> MSLSEIKHWVFDMDGTLTIAVHDFAAIREALSIPAEDDILTHLAALPADESAAKHAWLLEHERDLAQGSRPAPGAVELVRELAGRGYRLGILTRNARELAHVTLEAIGLADCFAEADVLGRDEAPPKPHPGGLLKLAEAWDVSPSRMVMVGDYRFDLDCGRAAGTRTVLVNLPDNPWP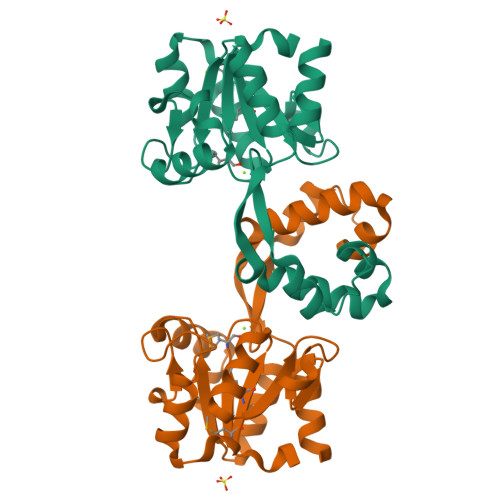ELTDWHARDCAQLRDLLSAEGHHHHHH> GAACGACACTGA;> CGTCGACTC;> TCAACG;> TCGAGTCGGTGTCGT

In this work, we exhaustively probe the ability of all 36 immobile HJ sequences to form DNA crystals in two different designed systems. Three separate self-assembling DNA crystal systems are described in this report: the “4 × 5” and “4 × 6” designs (collectively referred to as the 4 × N systems), and a third construct with a “scrambled” sequence variant of the 4 × 6 lattices. Self-assembly was mediated by three constituent oligonucleotides: (S1) containing four sequence repeats of either 5 or 6 bases; (S2) composed of 21 bases containing complementary regions to both (S1); and (S3) which forms the second junction crossover. The HJ serves as the fundamental component at the core of each unit, and the ultimate assembly of the full lattice is facilitated by the complementary 2-base sticky ends that tail each duplex.

To investigate this possibility, we designed “scrambled” sequences with targeted base substitutions, while maintaining GC content, along each “stem”. Contrary to the buffer preference observed with the native P32 crystals, the scrambled systems exhibited an exclusive preference towards low salt buffers, much like the native R3 crystals. Remarkably, only J1 and J2 retained the P32 symmetry, with all others yielding an R3 lattice. The average angles of the R3 and P32 crystals were 61.00° (σ = 1.21) and 58.05° (σ = 1.39), respectively. However, in the majority of the crystal structures reported here, the cacodylate anion indeed fits best into the electron density map of our X-ray structures, due to the presence of sodium cacodylate in the crystallization solution.> GPLGSPEFNRPVKRMIALYDYDPQELSPNVDAEQVELCFKTGEIILVYG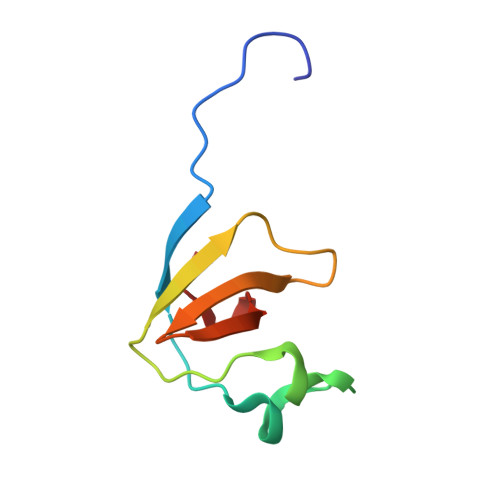DMDEDGFYMGELDGVRGLVPSNFLAD>[2x]GAMEPLIDPYTQTNAVSYERFIRWYSKENHISATTEDLYNSLHGTYNNYKQDLYARTARSFVESHCDEAWFEDSYWVDESQGRVLEVSENEKSYRRALYDKFMDRLDAGYYDDFQLPTAE;>[2x]MEMPQLSKWNQDSRNDAMENTLLVSHVLPNISVAQIHNALDGISFVQHFSLSTINLIKNDERSLWVH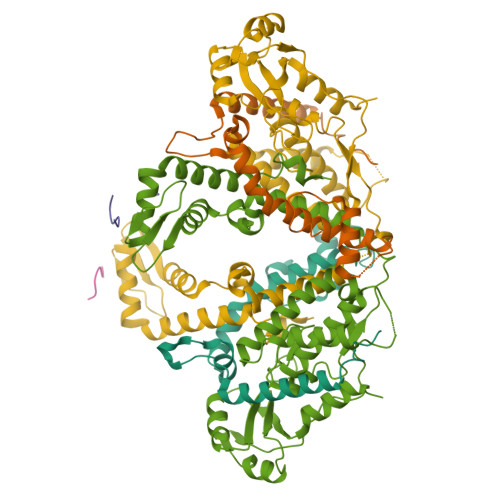FKAGTNMDGAKEAVDGIQLDSNFTIESENPKIPTHTHPIPIFEIASSEQTCKNLLEKLIRFIDRASTKYSLPNDAAQRIEDRLKTHASMKDDDDKPTNFHDIRLSDLYAEYLRQVATFDFWTSKEYESLIALLQDSPAGYSRKKFNPSKEVGQEENIWLSDLENNFACLLEPENVDIKAKGALPVEDFINNELDSVIMKEDEQKYRCHVGTCAKLFLGPEFVRKHINKKHKDWLDHIKKVAICLYGYVLDPCRAMDPKVVSSAWSHPQFEK;>KNEEDESNDSDKEDGEISEDD[2x]>[4x]MDQKPQPAKTHATEVTVLEGKTMGTFWRASIPGIDAKRSAELKEKIQTQLDADDQLLSTYKKDSALMRFNDSQSLSPWPVSEAMADIVTTSLRIGAKTDGAMDITVGPLVNLWGFGPEQQPVQIPSQEQIDAMKAKTGLQHLTVINQSHQQYLQKDLPDLYVDLSTVGEGYAADHLARLMEQEGISRYLVSVGGALNSRGMNGEGLPWRVAIQKPTDKENAVQAVVDINGHGISTSGSYRNYYELDGKRLSHVIDPQTGRPIEHNLVSVTVIAPTALEADAWDTGLMVLGPEKAKEVVRREGLAVYMITKEGDSFKTWMSPQFKSFLVSEKNLEHHHHHH

We recently reported a flavin‐trafficking protein (Ftp) in the syphilis spirochete Treponema pallidum (Ftp_Tp) as the first bacterial metal‐dependent FAD pyrophosphatase that hydrolyzes FAD into AMP and FMN in the periplasm. Orthologs of Ftp_Tp in other bacteria (formerly ApbE) appear to lack this hydrolytic activity; rather, they flavinylate the redox subunit, NqrC, via their metal‐dependent FMN transferase activity. In the current study, we identified a bimetal center in the crystal structure of Escherichia coli Ftp (Ftp_Ec) and show via mutagenesis that a single amino acid substitution converts it from an FAD‐binding protein to a Mg2+‐dependent FAD pyrophosphatase (Ftp_Tp‐like). A high‐resolution structure of the Ftp‐mediated flavinylated protein of Shewanella oneidensis NqrC identified an essential lysine in phosphoester‐threonyl‐FMN bond formation in the posttranslationally modified flavoproteins.

Therefore, we conducted extensive crystallization screening of Ftp_Ec wild‐type protein reconstituted in vitro with Mg2+ and FAD in an attempt to obtain a crystal structure of FAD and metal ions bound to the enzyme. There are four monomers in the asymmetric unit of each crystal structure, and the r.m.s.d. of the monomers within each structure ranges from 0.5 to 1.6 Å and 0.3 to 1.6 Å, respectively, between the two structures for approximately 300 Cα carbons. John Wiley & Sons, LtdIn the site previously denoted in the Ftp_Tp structure as metal binding site 1, a single metal ion is bound in the wild‐type and Ftp_EcE169K protein variant structures. Aided by the high resolution of our structural data, two water molecules were observed bound to each metal ion and thus the coordination number for the metal is seven, consistent with a Ca2+ rather than a Mg2+ ion as observed in the Ftp_Tp structures. Refinement of the metal in this site as a Mg2+ ion resulted in large positive peaks in a difference electron‐density map; these peaks disappeared when modeled as a Ca2+ ion. Thus, in agreement with the original structure determination, we have assigned these as Ca2+ ions. Superposition of three representative Ftp_Ec monomers illustrates the inherent flexibility of the loop region near the active site comprising residues 237–253. The Ftp_Ec structures suggest that in solution the cores of the Ftp enzymes remain stable, whereas a single flexible loop adopts different conformations during the catalytic cycle. Recombinant wild‐type Ftp_Ec was able to flavinylate RnfG_Ec in a Mg2+‐dependent manner in the presence of FAD (lane 4), suggesting that this type of posttranslational flavinylation reaction indeed is a protein‐dependent FMN transferase activity, rather than an autocatalytic one.> GSQNTANTGISNSNLNTTTTRKNIQSRNWYLSDSQWAAFKDDEITSTKHKNDYTDPHANKNIDKSALNIHADENDE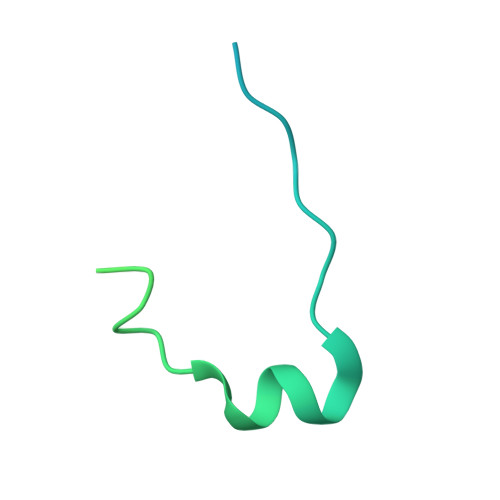GSVDNTLGSDRSNELEIRGKYVVVPETSQDMAFK>[7x]XG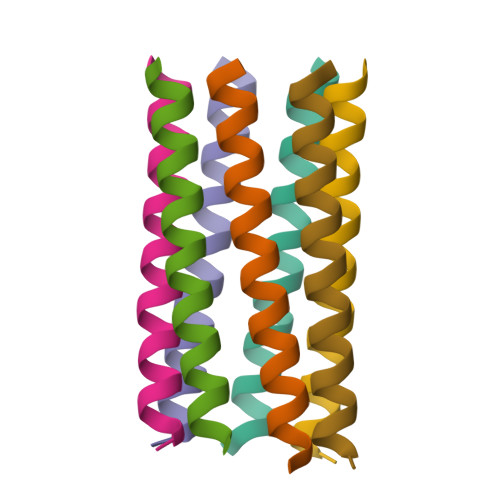EIAKALREIAKALRECAWAHREEAKALRG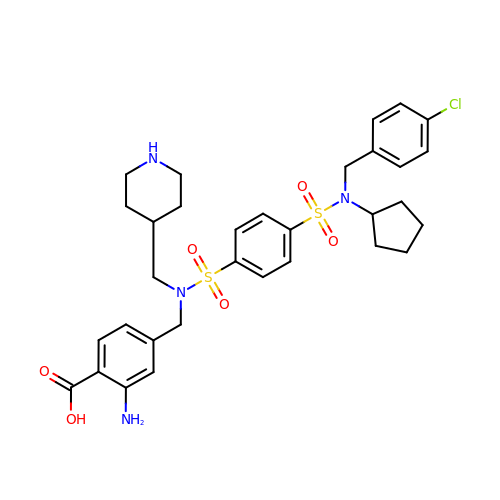2-azanyl-4-[[[4-[(4-chlorophenyl)methyl-cyclopentyl-sulfamoyl]phenyl]sulfonyl-(piperidin-4-ylmethyl)amino]methyl]benzoic acid | C32 H39 Cl N4 O6 S2 | AJWFYWFNVBQYRG-UHFFFAOYSA-N4-[7-(3,3-dimethylbut-1-yn-1-yl)naphthalen-1-yl]-5-methoxy-2-methyl-2,4-dihydro-3H-1,2,4-triazol-3-one 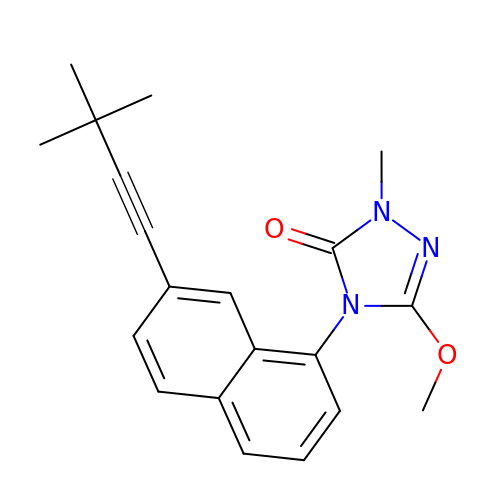| C20 H21 N3 O2 | XLOATFKILHMZGY-UHFFFAOYSA-N Long-term immune evasion by the African trypanosome is achieved through repetitive cycles of surface protein replacement with antigenically distinct versions of the dense Variant Surface Glycoprotein (VSG) coat. The mature VSG proteins are attached to the cell surface by a GPI-anchor, and consist of two main regions: (1) a large, N-terminal domain (NTD) of roughly 300–400 amino acids that is most distal to the membrane and (2) a smaller, membrane-proximal C-terminal domain (CTD) spanning 80–120 amino acids beneath the NTD that harbors the GPI-anchor. Therefore, at the heart of antigenic variation in the African trypanosome are the NTDs of the VSGs. These large subdomains are elongated folds centered on a three-helix bundle scaffold.

The structures of VSG21 and VSG545 were also determined, both harboring closely related folds and biochemical properties that distinguish them from other VSGs. Of note is the fact that both structures were obtained with proteolytic removal of the bottom lobe (contained in the C-terminal region of the NTD sequence). This cleavage occurred spontaneously during crystallization experiments performed with full-length VSG21 and the NTD of VSG545 that had been produced by limited proteolysis with Endoproteinase Lys-C (LysC). Presumably these cleavage events in the crystallization experiments occurred from residual contaminating endogenous protease(s) from T. brucei (and/or possibly residual LysC for VSG545). In contrast, for VSG21 and VSG545, the cleavage in the crystallization drops produced a truncated NTD missing the bottom lobe sequence but maintaining the 3-helix bundle and top lobe of the protein. Finally, it should be noted that for VSG545, crystals were only obtained with PNGase treated material, removing the N-linked glycan. VSG21 and VSG545 are more similar to each other than these other VSGs, however, distinguished from them by the tightly twisted nature of the top lobe and, directly beneath it, the presence of a second three-stranded beta-sheet perpendicular to the axis of the 3-helix bundle. VSG21 and VSG545 align well to each other in the top lobe but not to the other VSGs with beta-sheet top lobes. Superpositions with predicted models from AlphaFold (which were accurate enough to solve the experimental structures by molecular replacement) show possible conformations of the full NTD for each protein.

>MRKTRYIQEGTVSLALLPALVVSAGIPLHNRKAQINTPCDASHYAAAVADNAVSAFEQALGRAQDATVAANKLHLLASKLAGAQKAATTILAAAAGAAAADAIQKIAAATPNFAKGFAALNEIKGGQIIVDEMLKSKIEDAATVAAASSTSGATIVKIKPKLQPATKRACHDEQGKPTKTQDKAVEVAGDITLTLFSLKAETPGTTTDQKLTLCGHGSPSQDPATASCQNSQANLGIKGGSFIVKHQMQTTRTTTGATASYSAIASEDTVPNGDTITAQLTEIAKLENAVQALQNVHESAEAKSLAGKSDIKEVVARALAGETASYADTKIQKQVDGFLEAVFGKDASTVTGVIVKELKDLIPPKVAFSGAGNTKLEEITDPNQIADATTYYTVRSYIADQEEKNKSSTSPSCTTKTEKAKEPAKTTDECKKHTTNDACKKEKGCDFDEKKDPKCFPKVETEKKDEKSFSSNLRVSVPQVFAAFAALLF[2x]>MPKIQTYVNNNVYEQITDLVTIRKQEGIEEASLSNVSSMLLELGLRVYMIQQEKREGGFNQMEYNKLMLENVSRVRAMCTEILKMSVLNQESIASGNFD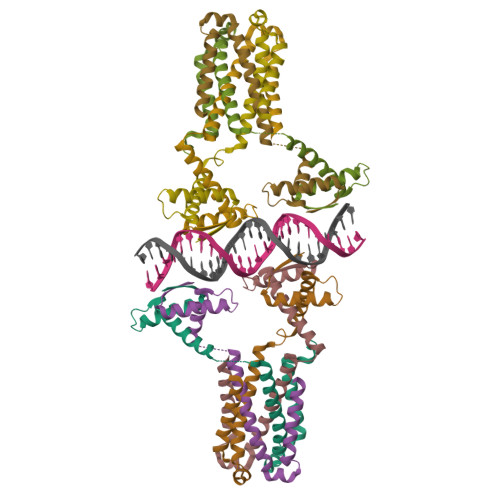YAVIKPAIDKFAREQVSIFFPDDEDDQE[4x]>MKLKSFGVFGNPIKHSKSPLIHNACFLTFQKELRFLGHYHPILLPLESHIKSEFLHLGLSGANVTLPFKERAFQVCDKIKGIALECGAVNTLVLENDELVGYNTDALGFYLSLKQKNYQN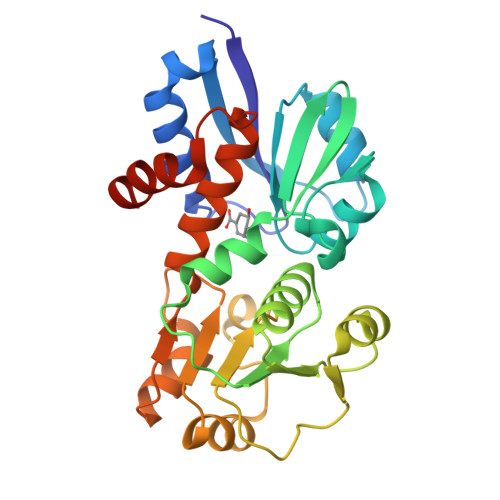ALILGAGGSAKALACELKKQGLQVSVLNRSSRGLDFFQRLGCDCFMEPPKSAFDLIINATSASLHNELPLNKEVLKGYFKEGKLAYDLASGFLTPFLSLAKELKTPFQDGKDMLIYQAALSFEKFSASQIPYSKAFEVMRSVFLEHHHHHH[2x]The long interspersed nuclear element-1 (LINE-1 or L1) retrotransposon is the only active autonomously replicating retrotransposon in the human genome. To insert a new copy into the genome, L1 uses target-primed reverse transcription (TPRT). The EN initiates this pathway by creating a single-stranded nick in genomic DNA at the semi-specific 5′-TTTT*A-3′ consensus sequence, with the asterisk marking the location of the cleaved phosphodiester bond. Therefore, the EN plays a key role in beginning the process of creating and integrating a new L1 copy into the genome.

To aid our docking efforts, we solved two EN structures by x-ray crystallography. Previous structures of the wild-type EN at the time this work was completed did not contain bound catalytic metal ions. Since the EN requires either Mg2+ or Mn2+ for activity, we believe this provides a better representation of the electrostatic environment of the active site for docking than the apo structure (protein without a metal ion). Our previous attempts to screen compound libraries unbiased by AD2 used the apo EN structure and resulted in no compounds with in vitro efficacy. Second, we expanded the structural diversity of the compounds screened by using the structure of EN bound to Mn2+ instead of the apo structure, and were able to find additional inhibitors using LeDock and AutoDock Vina by screening ZINC subsets, including FDA and internationally approved drugs. Therefore, we used the structure of the EN bound to Mn2+ for docking of Groups 2, 3, and 4. For example, the structurally analogous site to the EN S202 is the APE1 W280, which decreases the size of the APE1 binding surface relative to the EN. In our molecular docking experiments, we included the full EN DNA binding site (area used for docking is shown in Supplementary Fig. 1a) to maximize potential interactions with candidate compounds and opportunities for specificity relative to APE1.

>[2x]MTGSTSHITILTLNINGLNSAIKRHRLASWIKSQDPSVCCIQETHLTCRDTHRLKIKGWRKIYQANGKQKKAGVAILVSDKTDFKPTKIKRDKEGHYIMVKGSIQQEELTILNIYAPNTGAPRFIKQVLSDLQRDLDSHTLIMGDFNTPLSTLDRSTRQKVNKDTQELNSALHQADLIDIYRTLHPKSTEYTFFSAPHHTYSKIDHIVGSKALLSKCKRTEIITNYLSDHSAIKLELRI> GGSQTVTGGLRSLYQRKVLPLEEAYRFHEFHSPALEDADFENKPMILLVGQYSTGKTTFIRYLLEQDFPGMRIGPEPTTDSFIAVMYGETEGSTPGNALVVDPKKPFRKLSRFGNAFLNRFMCSQLPNQVLKSISIIDSPGILSGEKQRISRGYDFCQVLQWFAERVDRIILLFDAHKLDISDEFSEAIKAFRGQDDKIRVVLNKADQVDTQQLMRVYGALMWSLGKVINTPEVLRVYIGSFWAQPLQNTDNRRLFEAEAQDLFRDIQSLPQKAAVRKLNDLIKRARLAKVHAYIISYLKKEMPNM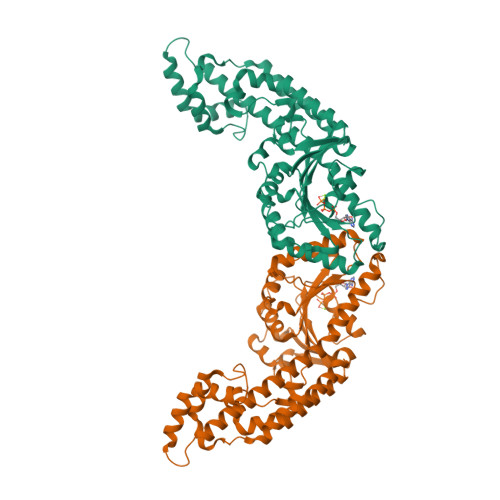FGKENKKRELIYRLPEIYVQLQREYQISAGDFPEVKAMQEQLENYDFTKFHSLKPKLIEAVDNMLTNKISSLMGLISQEEMNMPTQMVQGGAFDGTTEGPFNQGYGEGAKEGADEEEWVVAKDKPVYDELFYTLSPINGKISGVNAKKEMVTSKLPNSVLGKIWKLADCDCDGMLDEEEFALAKHLIKIKLDGYELPNSLPPHLVPPSHRKSLPKAD> MLSKKFGLSM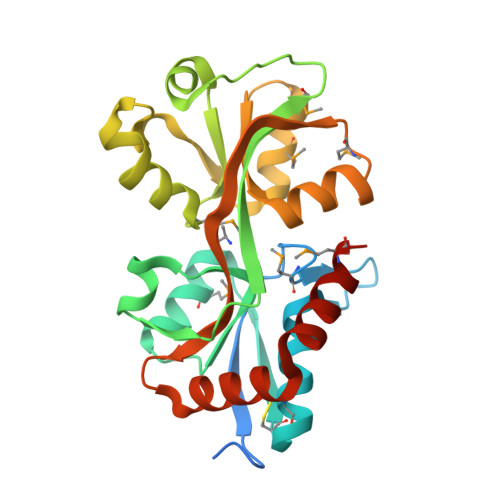IVLGIMSSSAFADSIVEGRTLNVAVSPASPPMLFKSADGKLQGIDLELFSSYCQSRHCKLNITEYAWDGMLGAVASGQADVAFSGISITDKRKKVIDFSEPYYINSFYLVSMANHKITLNNLNELNKYSIGYPRGMAYSDLIKNDLEPKGYYSLSKVKLYPTYNETMADLKNGNLDLAFIEEPVYFTFKNKKKMPIESRYVFKNVDQLGIAFKKGSPVRDDFNLWLKEQGPQKISGIVDSWMKHHHHHH> VPA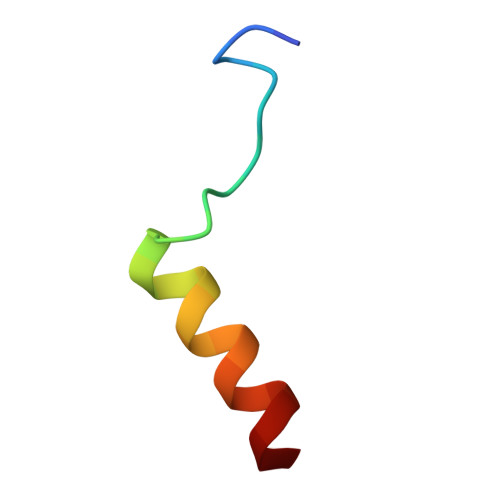NATGRALNDPREKRRLQREAER> QNVSLQPPPQQLIVQNKTIDLPAVYQLNGGEEANPHAVKVLKELLSGKQSSKKGMLISIGEKGDKSVRKYSRQIPDHKEGYYLSVNEKEIVLAGNDERGTYYALQTFAQLLKDGKLPEVEIKDYPSVRYRGVVEGFYGTPWSHQARLSQLKFYGKNKMNTYIYGPKDDPYHSAPNWRLPYPDKEAAQLQELVAVANENEVDFVWAIHPGQDIKWNKEDRDLLLAKFEKMYQLGVRSFAVFFDDISGEGTNPQKQAELLNYIDEKFAQVKPDINQLVMCPTEYNKSWSNPNGNYLTTLGDKLNPSIQIMWTGDRVISDITRDGISWINERIKRPAYIWWNFPVSDYVRDHLLLGPVYGNDTTIAKEMSGFVTNPMEHAESSKIAIYSVASYAWNPAKYDTWQTWKDAIRTILPSAAEELECFAMHNSDLGPNGHGYRREESMDIQPAA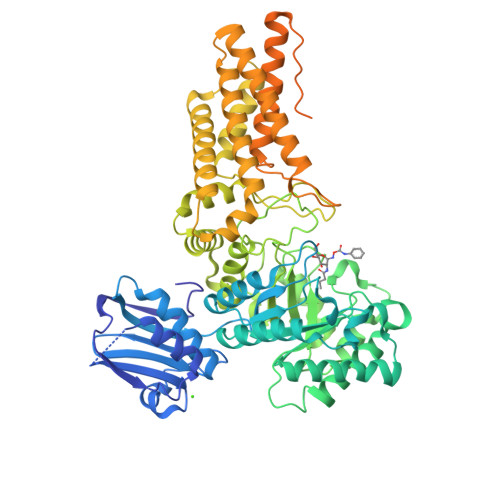ERFLKAFKEGKNYDKADFETLQYTFERMKESADILLMNTENKPLIVEITPWVHQFKLTAEMGEEVLKMVEGRNESYFLRKYNHVKALQQQMFYIDQTSNQNPYQPGVKTATRVIKPLIDRTFATVVKFFNQKFNAHLDATTDYMPHKMISNVEQIKNLPLQVKANRVLISPANEVVKWAAGNSVEIELDAIYPGENIQINFGKDAPCTWGRLEISTDGKEWKTVDLKQKESRLSAGLQKAPVKFVRFTNVSDEEQQVYLRQFVLTIEKK> XGACEA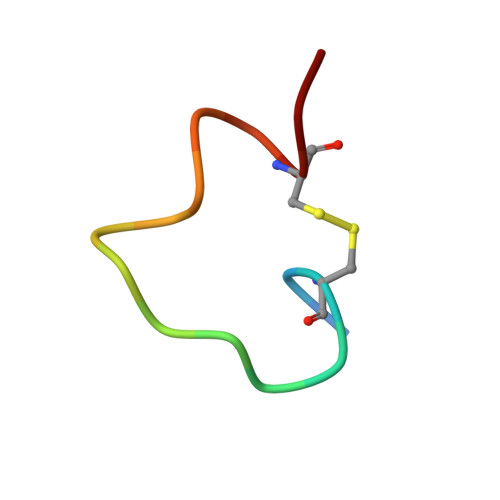RHREWAWLCAA>[3x]MATKGTKRSYEQMETDGERQNATEI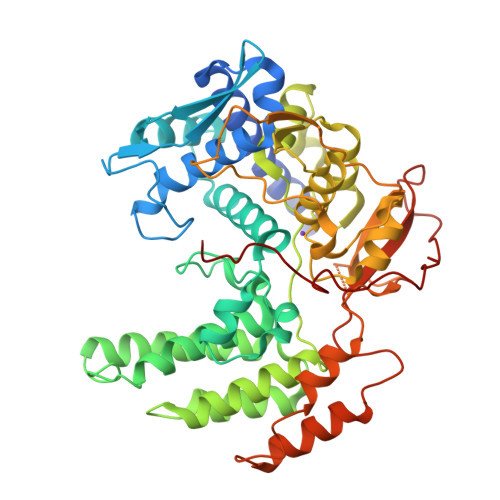RASVGKMIDGIGRFYIQMCTELKLSDYEGRLIQNSLTIERMVLSAFDERRNKYLEEHPSAGKDPKKTGGPIYRRVDGKWRRELILYDKEEIRRIWRQANNGDDATAGLTHMMIWHSNLNDATYQRTRALVRTGMDPRMCSLMQGSTLPRRSGAAGAAVKGVGTMVMELIRMIKRGINDRNFWRGENGRRTRIAYERMCNILKGKFQTAAQRTMVDQVRESRNPGNAEFEDLIFLARSALILRGSVAHKSCLPACVYGSAVASGYDFEREGYSLVGIDPFRLLQNSQVYSLIRPNENPAHKSQLVWMACHSAAFEDLRVSSFIRGTKVVPRGKLSTRGVQIASNENMETMESSTLELRSRYWAIRTRSGGNTNQQRASSGQISIQPTFSVQANLPFDRPTIMAAFTGNTEGRTSDMRTEIIRLMESARPEDVSFQGRGVFELSDEKATSPIVPSFDMSNEGSYFFGDNAEEYDN>PVMHPHGVP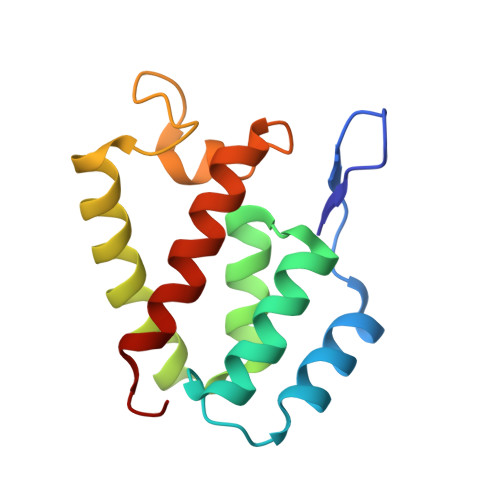PSHRPWQMKDLQAIKQEVSQAAPGSPQFMQTIRLAVQQFDPTAKDLQDLLQYLCSSLVASLHHQQLDSLISEAETRGITGYNPLAGPLRVQANNPQQQGLRREYQQLWLTAFAALPGS[2x]>[2x]ENSHLQSPKNTNKIEVLNWEAFSKKLKDYSSDQRQFHVLKLGFENRLGTLSTREELEEFGKNNNFLVINGKVTQNIHDFPHILVMNKGDVIAHNEEDYHNQMRELRFSGNGDLHNSMEPKRIHALFKIELDSNKRQLLNAAG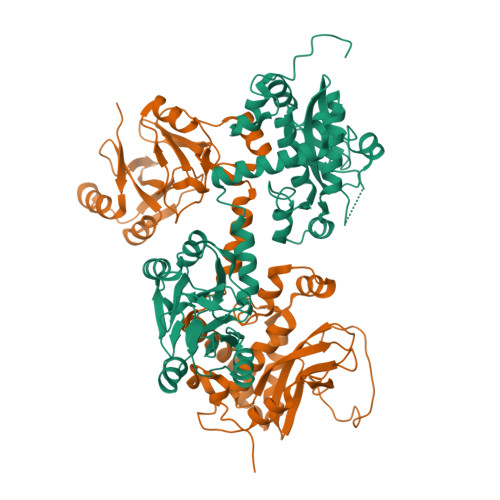LGTAENSLKNINGMTIYSHGLTVDNKYYEDYSKYTHNSVKNINVTKERFIANDDLIHKLIESSEAMKQSSERDKVKAFVQYVANHTTYDWEAANKAVQNYADINYYLGSDLFAVTERQKAMCVGFSTTAARAFNMLGLPAYVVVGKNAEGVPHATARVYYDKKWHTIDGTGFITGNKHQRSAKYSEKHFSTIGEDSYDVVEAGQEPKAERNYMIIDSNYESWAMKQKTADLLLFNKEKSLVGLDYIAYVEPTYITEN>MTGQAAPNLHTNILNRIANELALTYQGVFSAETINRYIFESYVSLARTAKIHTHLPILAEGFAKDRLHALAVAEGKVASPVPQVLFICVHNAGRSQIASALLSHYAGSSVEVRSAGSLPASEIHPLVLEI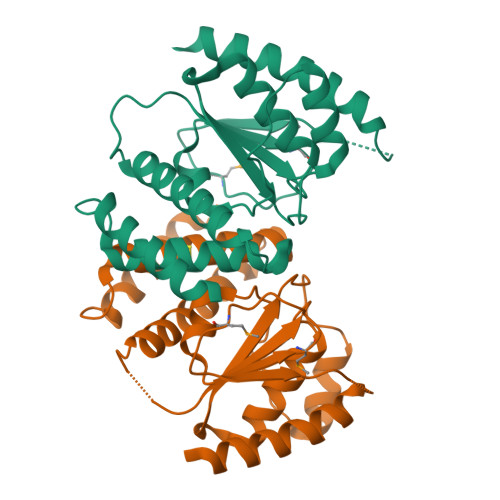LSERGVNISDAFPKPLTDDVIRASDYVITMGCGDVCPMYPGKHYLDWELADPSDEGEDKIQEIIEEIDGRIRELWKSIQLSQN[2x]> MHSTNNNSNKRNNEEKHKQPEIDSSANNGEGTSGTRAQTVGDTATEAGVRNETEAGASTRRQTDGTGLSGTNAKIATASSARQADVEKPADVTFTIENVDDVGIMQQKKPPTVVQSRTDVFNEQFANEALHPTTKVIFNGLDVNTEVQPLSDDFKQISDPKGYLTYSVKYEDQFTKKDKLRASEADDRIVGPTVNLFKYGAAVVNIDLNRDFFDTATGIDLTKGIPLVQDLLVPIGVTAGAEQSAEYVSGLLMVLFKVMTDNRLVIVGETTTPMSNTLSTVVNNVLRTTYHNNVGVNPALLRDFTQVNWLNRDITNMLQQAGTKYGLGLTETRLDYVRLVKTIVGHALNIDHFAASVLNINLRALMEANVTADDRIKALQAHSMISTQFHGPNQGALRPELAFDHDHIIRCLMLAAANYPRLEGIIVQINTGYVASANVIRPVSEKRYFPENLEQNQSAARLVSAVKARASEADISSIHLAIAREVSPMFNVHELKKIAESFEDPSSIVVVLEFILFALFFPTEFNRIKGDIQNVLLLFFSRWYPVEYGIFVQRGATYTINAAGEFEFSGRNEKWDQALYLSEHFPALFSDVPLAGANTIIAIMRLFTPQGFLRTDDLAIAANFPRASRNPQTYIPYTNQRGTVTNEFASRFRTIVATLANVVNERAVQDDMQKATRSCTKQWLRHLETQFDNIAVAHTDHLSVVYATMSNFMLNFTNNFSGNHATFKPDQYVITSPEGSYKPIIERQGETVDGLTIIDTSIVWPILCQCTYPLVRQSGKGVDAVSIMEEIVYPDPSTTLSQSLSVAQVLSKLTLPDAFINMILSGGDSVVMRTYQTEADDDLDEGIRMTTYDQYLSHIRERLHITNVPDPIYITGASTPDQIAASVQATHVAVVLYQSGVINGPASTYLRENEVLVVMPDYYDVVSRFANANLQMNNNRYHESVLEIADIFDQADFIQTSDAVRQLRALMPTLSTSQIRHAIERIAQITDVDSTDYGKLTLRFLGTLTRSLKMQNAQIRRIRPDGTVLRYDDQIDIEAFRWSRYFLDEL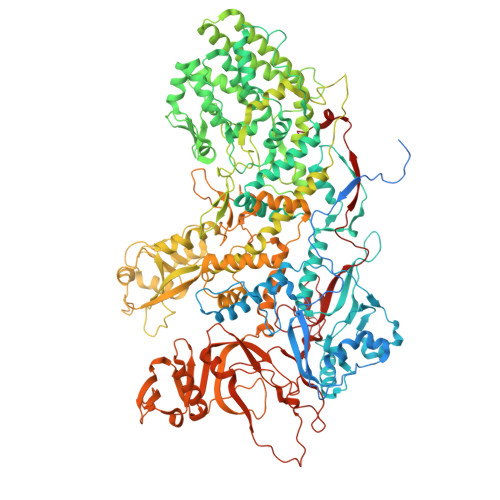QLRRLSVGLRLITNPRIARRFNGVRIMYLTDDDPDPDFVPDVPEGYVAVQYAHRLFSSSLANKRNRVTYTHPPTGMAYPSPTGRPHVHMTINERAGMSKLVADNIIASVIKSNWVVDILDIEYTAEVMTPSEGYTQHVDAESIMTAPKGKLFHLQFMDGLLRPEPSAFDPPASGEDMRLIYPLQPISVARSMRAIVNHNEVDRPRGAVAPSSYEMDTGTLSRNGDLLYSPVANGQVGIPKLEVDHISFSNVVSMMTANIRTGDDMAVERVNPDDVRAINIRNA> SRSGSDICSLPVLAKICQKIKLAMEQSVPFKDVDSDKYSVFPTLRGYHWRGRDCNDSDESVYPGRRPNNWDVHQDSNCNGIWGVDPKDGVPYEKKFCEGSQPRGIILLGDAAGAHFHISPEWITASQMSLNSFINLPTALTNELDWPQLSGATGFLDSTVGIKEKSIYLRLWKRNHCNHRDYQNISRNGASSRNLKKFIESLSRNKVLDYPAIVIYAMIGNDVCSGKSDPVPAMTTPEKLYSNVMQTLKHLNSHLPNGSHVILYGLPDGTFLWDNLHNRYHPLGQLNKDMTYAQLYSFLNCLQVSPCHGWMSSNKTLRTLTSERAEQLSNTLKKIAASEKFTNFNLFYMDFAFHEIIQEWQKRGGQPW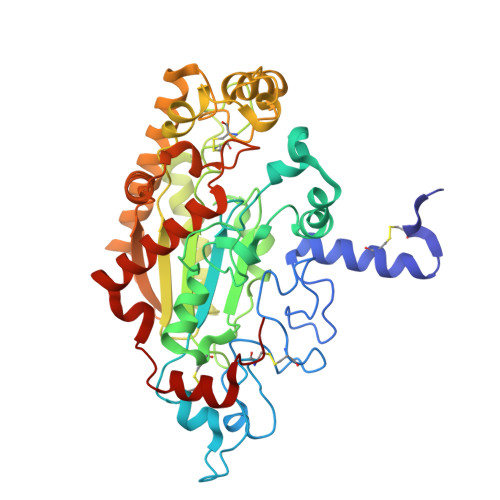QLIEPVDGFHPNEVALLLLADHFWKKVQLQWPQILGKENPFNPQIKQVFGDQGGH(3R)-3-cyclopentyl-3-[4-(7H-pyrrolo[2,3-d]pyrimidin-4-yl)-1H-pyrazol-1-yl]propanenitrile | C17 H18 N6 | 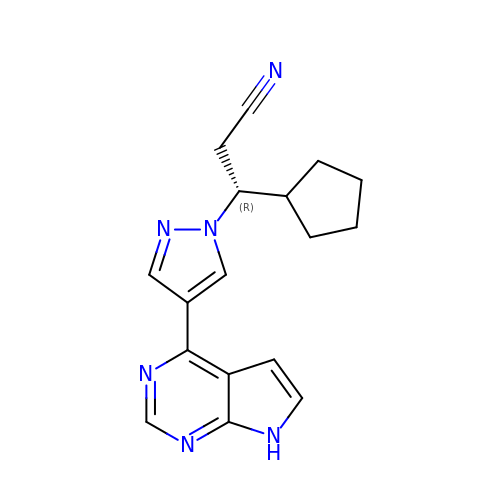HFNKQEVNSGCOJV-OAHLLOKOSA-N3'-AZIDO-3'-DEOXY-THYMIDINE-5'-ALPHA BORANO TRIPHOSPHATE | C10 H17 B N5 O12 P3 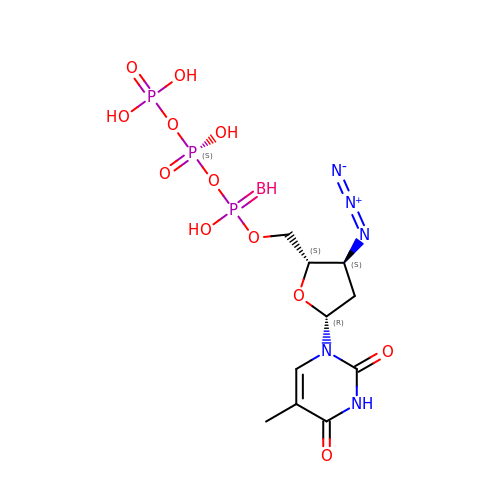| YRFDNFJEDDBNDW-NYNRLPRQSA-N>[2x]GMEQKLYKNYADDIAHYLKQGKKNNLQKGLSYEHFSKN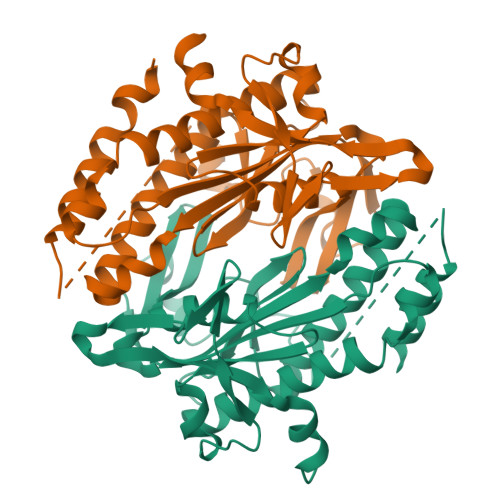LSSHPKMQWVDKTKNEANFRSLSALNTITGQITKYEEKLGAHPSFSHLKNTNDSEYHYIVSMFVDVRNSTGLFKKFDPDVVANICRTIQLATIHTCWYFDGYVHRLQGDGLMVYFGGKGTTKQKAVDNALMAASFISYFVKNDLKNLFEEQGVSRIYTRIGLDFGDDEDTLWHNAGIGECSEVTTTSLHTSLACKMQAQAESNGVVVGDNILPYKSSDKNYFTYKKYKKNGSELPYVYEIPEEYFRYKQHDFNWEKFLKNHPQIQEDEDGNLTFINPSLPPNPRVQQNINHLQQNVSGYKPYLR(2S,4S,5S)-5-amino-N-(3-amino-2,2-dimethyl-3-oxopropyl)-6-[4-(2-chlorophenyl)-2,2-dimethyl-5-oxopiperazin-1-yl]-4-hydroxy-2-(propan-2-yl)hexanamide | C26 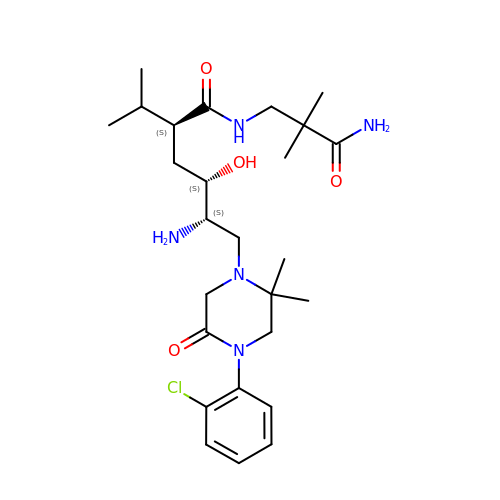H42 Cl N5 O4 | RBIIKVXVYVANCQ-CUWPLCDZSA-N PYRIMIDIN-2-AMINE | C4 H5 N3 | 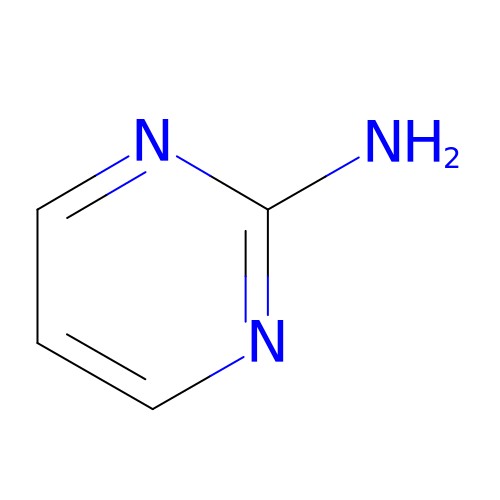LJXQPZWIHJMPQQ-UHFFFAOYSA-N> GSAMDNDHLVIEANIN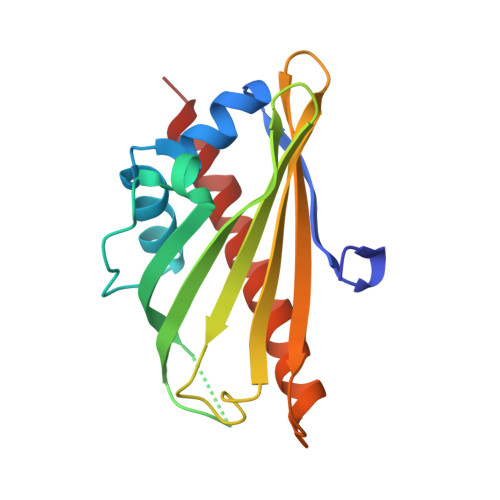APLGKVVNLLYGEDVSYYERILKAQKNFEISPIPNNFLTKKIRDYAYTKPLSGSIGPSKTKCLITDTLEHYDLEDYVKVLSITKNPDVPSGNIFSVKTVFLFSWDKNNSTKLTVYNSVDWTGKSWIKSMIEKGTFDGVADTTKIMISEIKKILSD>[2x]MSVDYPRDLIGYGSNPPHPHWP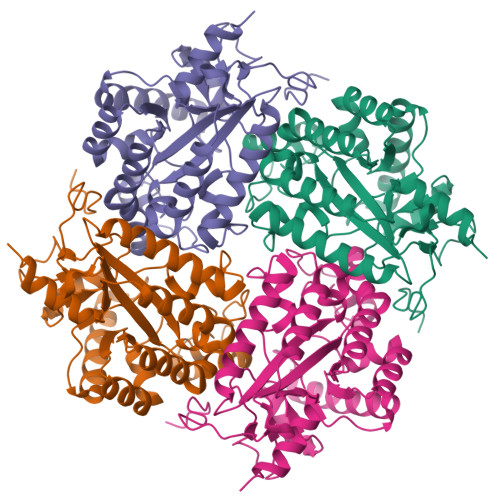GKARIALSFVLNYEEGGERNILHGDKESEAFLSEMVSAQPLQGERNMSMESLYEYGSRAGVWRILKLFKAFDIPLTIFAVAMAAQRHPDVIRAMVAAGHEICSHGYRWIDYQYMDEAQEREHMLEAIRILTELTGERPLGWYTGRTGPNTRRLVMEEGGFLYDCDTYDDDLPYWEPNNPTGKPHLVIPYTLDTNDMRFTQVQGFNKGDDFFEYLKDAFDVLYAEGAEAPKMLSIGLHCRLIGRPARLAALQRFIEYAKSHEQVWFTRRVDIARHWHATHPYTGAAK>[6x]MNKLVGLLVSSLFLASILIGIAPAITTTALTPPVSAGGIQAYLLTGSGAPASGLVLFVVNVSNIQVSSSNVTNVISTVVSNIQINAKTENAQTGATTGSVTVRFPTSGYNAYYDSVDKVVFVVVSFLYPYTTTSVNIPLSYLSKYLPGLLTAQPYDETGAQVTSVSSTPFGSLIDTSTGQQILGTNPVLTSYNSYTTQANTNMQEGVVSGTLTSFTLGGQSFSGSTVPVILYAPFIFSNSPYQAGLYNPMQVNGNLGSLSSEAYYHPVIWGRALINTTLIDTYASGSVPFTFQLNYSVPGPLTINMAQLAWIASINNLPTSFTYLSYKFSNGYESFLGIISNSTQLTAGALTINPSGNFTINGKKFYVYLLVVGSTNSTTPVEYVTKLVVEYPSSTNFLPQGVTVTTSSNKYTLPVYEIGGPAGTTITLTGNWYSTPYTVQITVGSTPTLTNYVSQILLKAVAYEGINVSTTQSPYYSTAILSTPPSEISITGSSTITAQGKLTATSASATVNLLTNATLTYENIPLTQYSFNGIIVTPGYAAINGTTAMAYVIGALYNKTSDYVLSFAGSQEPMQVMNNNLTEVTTLAPFGLTLLAPSVPATETGTSPLQLEFFTVPSTSYIALVDFGLWGNLTSVTVSAYDTVNNKLSVNLGYFYGIVIPPSISTAPYNYQNFICPNNYVTVTIYDPDAVLDPYPSGSFTTSSLPLKYGNM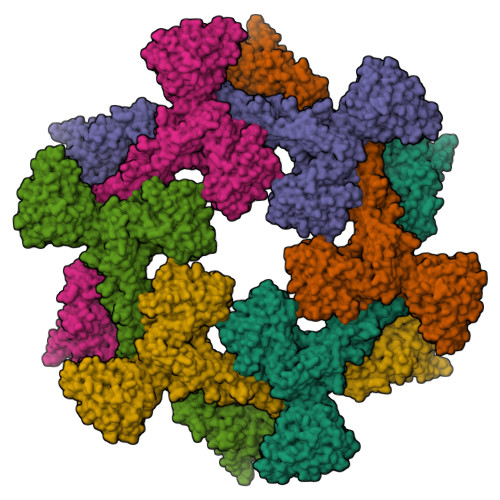NITGAVIFPGSSVYNPSGVFGYSNFNKGAAVTTFTYTAQSGPFSPVALTGNTNYLSQYADNNPTDNYYFIQTVNGMPVLMGGLSIVASPVSASLPSSTSSPGFMYLLPSAAQVPSPLPGMATPNYNLNIYITYKIDGATVGNNMINGLYVASQNTLIYVVPNGSFVGSNIKLTYTTTDYAVLHYFYSTGQYKVFKTVSVPNVTANLYFPSSTTPLYQLSVPLYLSEPYYGSPLPTYIGLGTNGTSLWNSPNYVLFGVSAVQQYLGFIKSISVTLSNGTTVVIPLTTSNMQTLFPQLVGQELQACNGTFQFGISITGLEKLLNLNVQQLNNSILSVTYHDYVTGETLTATTKLVALSTLSLVAKGAGVVEFLLTAYPYTGNITFAPPWFIAENVVKQPFMTYSDLQFAKTNPSAILSLSTVNITVVGLGGKASVYYNSTSGQTVITNIYGQTVATLSGNVLPTLTELAAGNGTFTGSLQFTIVPNNTVVQIPSSLTKTSFAVYTNGSLAIVLNGKAYSLGPAGLFLLPFVTYTGSAIGANATAIITVSDGVGTSTTQVPITAENFTPIRLAPFQVPAQVPLPNAPKLKYEYNGSIVITPQQQVLKIYVTSILPYPQEFQIQAFVYEASQFNVHTGSPTAAPVYFSYSAVRAYPALGIGTSVPNLLVYVQLQGISNLPAGKYVIVLSAVPFAGGPVLSEYPAQLIFTNVTLTQ>MSATAATVPPAAPAGEGGPPAPPPNLTSNRRLQQTQAQVDEVVDIMRV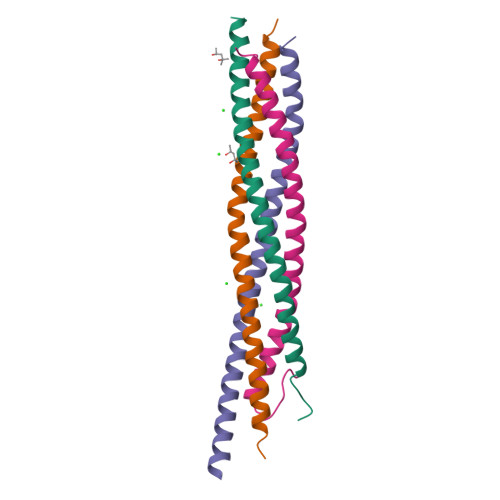NVDKVLERDQKLSELDDRADALQAGASQFETSAAKLKRKYWWKNLKMM[3x];>[3x]GIIMDSSISKQALSEIETRHSEIIKLENSIRELHDMFMDMAMLVESQGEMIDRIEYNVEHAVDYVERAVSDTKKAVKYQSKAR;>[3x]MAEDADMRNELEEMQRRADQLADESLESTRRMLQLVEESKDAGIRTLVMLDEQGEQLDRVEEGMNHINQDMKEAEKNLKDLGK;>VVDEREQMAISGGFIRRVTNDARENEMDENLEQVSGIIGNLRHMALDMGNEIDTQNRQIDRIMEKADSNKTRIDEANQRATKMLGSG[3x]> ARTVVLITGCSSGIGLHLAVRLASDPSQSFKVYATLRDLKTQGRLWEAARALACPPGSLETLQLDVRDSKSVAAARERVTEGRVDVLVCNAGLGLLGPLEALGEDAVASVLEVNVVGTVRMLQAFLPDMKRRGSGRVLVTGSVGGLMGLPFNDVYCASKFALEGLCESLAVLLLPFGVHLSLIECGPVH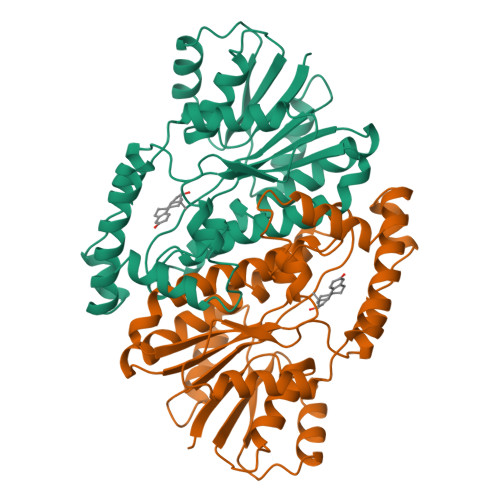TAFMEKVLGSPEEVLDRTDIHTFHRFYQYLAHSKQVFREAAQNPEEVAEVFLTALRAPKPTLRYFTTERFLPLLRMRLDDPSGSNYVTAMHREVFGDVPAKAEAGAEAGGGAGPGAEDEAGRSAVGDPELGDPPAAPQ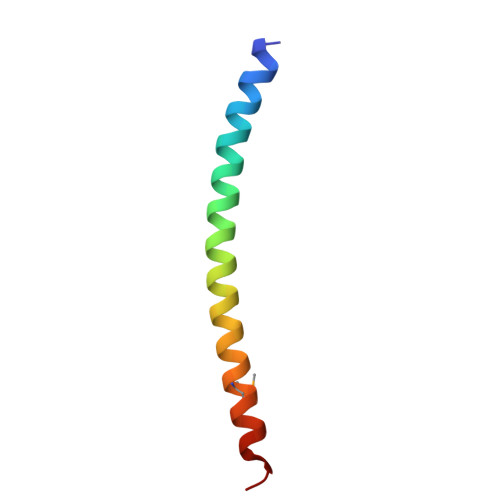> QQEIFDKQRRLQELSEKVRTCHQEISALRKALQEKEAEMLQVLEDIQTI CRL2KLHDC2 has been proposed as an attractive additional E3 ligase handle for targeted protein degradation. Specifically, KLHDC2 recognizes substrates possessing a Gly-Gly C-terminal degron (C-degron) sequence. First, crystal structures showed KLHDC2 binds substrate C-termini in a well-defined pocket lined by aromatic residues available to engage a ligand. Ligands were identified that engage the C-degron binding site in KLHDC2, subjected to structure-based improvement, and linked to JQ1 for BET-family neo-substrate recruitment.

However, the introduction of a nitrogen atom or disruption of aromaticity on the ring led to a loss of activity. This SAR campaign led to our first lead, SJ10278, with enhanced potency compared to SJ6145 as measured by SPR (Kd = 8.8 μM), competitive binding to a degron peptide (TR-FRET IC50 = 24.1 μM), and thermal shift (ΔTm = 3.5 °C). To understand how SJ10278 engages KLHDC2’s di-Gly binding pocket, we obtained a crystal structure at 1.95 Å resolution. Superposition with the structure of a di-Gly degron peptide confirmed the ligand targets KLHDC2’s substrate-binding pocket. The acid moiety of SJ10278 is stabilized by canonical contacts with KLHDC2’s R236, S269, and R241. The thiazole and chloro-phenyl moieties of SJ10278 contact adjacent hydrophobic and polar elements typically engaged by consensus degrons. Two features of the SJ10278-KLHDC2 co-crystal structure were notable for structure guided improvement of ligand potency. First, the constellation of hydrophobic residues surrounding the chloro-phenyl moiety suggested adding hydrophobic character to this portion of the ligand might improve binding. This is particularly evident in electrostatic representations of the binding pocket surface, which shows SJ10278 adjacent to a hydrophobic cleft in KLHDC2. Secondly, comparison to a bound consensus di-Gly substrate showed that binding of SJ10278 leaves space in the pocket. However, attempts to substitute the SJ10278 carboxylate with a sulfonate isostere led to a loss of activity.

>GSPAFESYESMELACPAERSGHVAVSDGRHMFVWGGYKSNQVRGLYDFYLPREELWIYNMETGRWKKINTEGDVPPSMSGSCAVCVDRVLYLFGGHHSRGNTNKFYMLDSRSTDRVLQWERIDCQGIPPSSKDKLGVWVYKNKLIFFGGYGYLPEDKVLGTFEFDETSFWNSSHPRGWNDHVHILDTETFTWSQPITTGKAPSPRAAHACATVGNRGFVFGGRYRDARMNDLHYLNLDTWEWNELIPQGICPVGRSWHSLTPVSSDHLFLFGGFTTDKQPLSDAWTYCISKNEWIQFNHPYTEKPRLWHTACASDEGEVIVFGGCANNLLVHHRAAHSNEILIFSVQP[2x]>[2x]AYTTFSQTKNDQLKEPMFFGQPVNVARYDQQKYDIFEKLIEKQLSFFWRPEEVDVSRDRIDYQALPEHEKHIFISNLKYQTLLESIQGRSPNVALLPLISIPELETWVETWAFSETIHSRSYTHIIRNIVNDPSVVFDDIVTNEQI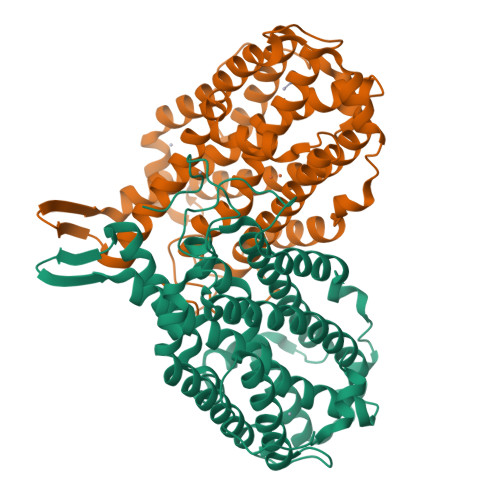QKRAEGISSYYDELIEMTSYWHLLGEGTHTVNGKTVTVSLRELKKKLYLCLMSVNALEAIRFYVSFACSFAFAERELMEGNAKIIRLIARDEALHLTGTQHMLNLLRSGADDPEMAEIAEECKQECYDLFVQAAQQEKDWADYLFRDGSMIGLNKDILCQYVEYITNIRMQAVGLDLPFNTRSNPIPWINTWLVSDNVQVAPQEVEVSSYLVGQIDSEVDTDDLSNFQL The intracellular c-di-GMP level is controlled by a dynamic balance of synthesis by diguanylate cyclases (DGCs, containing a GGDEF domain) and degradation by specific phosphodiesterases (PDEs, containing EAL or HD-GYP domains). In P. aeruginosa, the SiaA/B/C/D signaling network regulates biofilm and aggregate formation in response to environmental stimuli. Recently, we elucidated that the DGC activity of SiaD is modulated by its binding partner via direct interaction, whereas phosphorylation of SiaC by the kinase SiaB prevents the SiaC-SiaD interaction and activation of SiaD. Dynamic switching between the inactive pentamer and active dimer is regulated by SiaC: SiaC induces deoligomerization of the inactive SiaD pentamer and binds to the two conserved motifs in the stalk domain of the reconstructed active SiaD dimer to stabilize its conformation for further catalysis.

To investigate the regulation of SiaD by SiaC, we determined the crystal structure of full-length SiaD in complex with SiaC. In the asymmetric crystallographic unit, two SiaD and four SiaC molecules bind together, adopting a unique extensive conformation: two SiaD molecules (SiaD-A and SiaD-B) form a parallel coiled-coil via their stalk helices, and their dimeric stalks are stabilized by the binding of two pairs of SiaC molecules (SiaC-C/D, SiaC-E/F), each at distinct locations (proximal or distal to the SiaD DGC domain) along the dimeric stalk. In this complex, each the SiaD monomer consists of an N-terminal domain, a C-terminal DGC domain, and a long extended coiled-coil-like helical stalk domain linking the N- and C-terminal domains. The stalk and DGC domains of SiaD monomers bind each other in parallel, with a central C2 axis of symmetry, to form a dimer that covers one-third of the SiaD protein surface (4460 Å2 of 15,159 Å2). Two DGC domains in the complex are oriented anti-parallel, with their active sites facing each other. Moreover, a non-hydrolyzable GTP analog GpCpp molecule was observed to bind in the active site of SiaD-A. However, there was only one GpCpp molecule observed in one of the SiaD A-sites, leaving the other A-site empty. In addition, the side chain of the key residue T68ʹ in the N-terminal portion of the SiaC α2ʹ helix inserts into a space between the parallel SiaD stalk helices, forming strong hydrogen bonds with the side chains of SiaD residues S82 and Q86. Triple mutagenesis of N67ʹ, T68ʹ, and S69ʹ to alanine or phosphorylation of T68ʹ significantly prevents the binding of SiaC to SiaD.

>[2x]SMSRERELDAWIDGLLADPQFHGHPLHQALARLRQQSLEQLVRLERIARISDGFQSMAREQNLSLSERYHKQLRRLEKVARISDRYQQMMRDLNLALKEASIRDPLTGLPNRRMLLERLREENERSQRHGQSYVLAMLDVDFFKQVNDTWGHDSGDRVLVEIARAMESELREYDLCGRWGGEEFLLLLPQTRLQDAGPVLERVRDSVRTLAVRVGTEALSVTASVGVTEHRIGETYSQTVNRADAALLDAKRSGRDKCVFAALPPLPAPSRPAPAR;>SMSDLHIPGTQSTPAIQGDWQAGRLSMQGDSYPENSYELFGQVIDWVERFLADGQRPLELDLRLLYLNTSSIKAMMDILDLLEEAHQGGRPVSLRWHYDRRNERVAELAEEFREDCSFPFAIQAHDE[4x]> KSPIFGPEEVNSVEGNSVSITCYYPPTSVNRHTRKYWCRQGARGGCITLISSEGYVSSKYAGRANLTNFPENGTFVVNIAQLSQDDSGRYKCGLGINSRGLSFDVSLEVSQGPGLLNDTKVYTVDLGRTVTINCPFKTENAQKRKSLYKQIGLYPVLVIDSSGYVNPNYTGRIRLDIQGTGQLLFSVVINQLRLSDAGQYLCQAGDDSNSNKKNADLQVLKPEPELVYEDLRGSVTFHCALGPEVANVAKFLCRQSSGENCDVVVNTLGKRAPAFEGRILLNPQDKDGSFSVVITGLRKEDAGRYLCGAHSDGQLQEGSPIQAWQLFVNEESTIPRSPTVVKGVAGGSVAVLCPYNRKESKSIKYWCLWEGAQNGRCPLLVDSEGWVKAQYEGRLSLLEEPGNGTFTVILNQLTSRDAGFYWCLTNGDTLWRTTV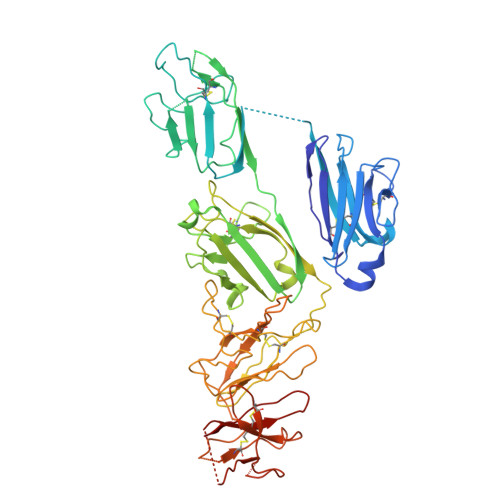EIKIIEGEPNLKVPGNVTAVLGETLKVPCHFPCKFSSYEKYWCKWNNTGCQALPSQDEGPSKAFVNCDENSRLVSLTLNLVTRADEGWYWCGVKQGHFYGETAAVY Sugars and other sweet-tasting compounds are detected by the sweet taste receptor, a member of the class C GPCR family. The sweet receptor is a heterodimer composed of TAS1R2 and TAS1R3,3,4 two type 1 taste receptor family members that share the distinctive architecture of class C GPCRs: a large extracellular Venus flytrap (VFT) domain, responsible for ligand recognition; a cysteine-rich domain (CRD); and a seven-transmembrane (7TM) domain that mediates G protein coupling. To address this gap, here we present cryo-electron microscopy (cryo-EM) structures of the sweet receptor in the inactive, unliganded state, as well as in the activated, sucralose- and advantame-bound states. Unlike other class C GPCRs, such as mGluR, CaSR and GABAB receptors, where agonists stabilize inter-subunit VFT interactions to promote activation, the sweet receptor is activated by the rearrangement of a TAS1R2 VFT loop, which destabilizes interactions between the lower VFT lobes and the VFT–CRD interfaces.

We first determined the structure of the human/mouse sweet receptor in the absence of sweeteners. To improve the resolution, we combined all particles to generate a global reconstruction at 3.1 Å resolution, then performed local refinement focused on the VFT/CRD region or the 7TM domain, obtaining final resolutions of 2.9 Å and 3.6 Å, respectively. In the unliganded (apo) state, TAS1R2 and TAS1R3 show a highly asymmetric architecture, and their extracellular domains are markedly tilted relative to the membrane plane. In our apo sweet receptor structure, the two subunits pack closely against each other at both the upper and lower lobes of the VFT domains, as well as at the 7TM domains. This sharply contrasts with the apo states of mGluRs and the calcium-sensing receptor (CaSR), where the dimer interface is restricted to the VFT upper lobes (LB1s), while the lower lobes (LB2s) and 7TM domains remain largely disengaged. The tight packing of the sweet receptor is facilitated by interactions between VFT domains and CRDs, with the VFT LB2s held together by loops extending from the CRDs. Phe519 and His520 from TAS1R3 CRD are wedged deeply into the cleft between the two LB2s, effectively clasping them together, whereas equivalent residues Ile510 and His511 from TAS1R2 also extend into the VFT layer. This configuration reinforces the dimer interface and would enable the VFT domain of one subunit to directly communicate with the CRD of the other subunit, potentially allowing efficient cross-subunit allosteric coupling. Notably, such an arrangement differs from other class C GPCRs, where the VFT layer and the CRD remain structurally separated.

> SDFYLPGDYLLGGLFSLHANMKGIVHLNFLQVPMCKEYEVKVIGYNLMQAMRFAVEEINNDSSLLPGVLLGYEIVDVCYISNNVQPVLYFLAHEDNLLPIQEDYSNYSSRVVAVIGPDNSESVMTVANFLSLFLLPQITYSAISDELRDKVRFPALLRTTPSADHHIEAMVQLMLHFRWNWIIVLVSNDTYGRDNGQLLGERVARRGICIAFQETLPTLQPNQNMTSEERQRLVTIVDKLQQSTARVVVVFSPDLTLYHFFNEVLRQNFTGAVWIASESWAIDPVLHNLTELRHLGTFLGITIQSVPIPGFSEFREWGPQAGPPPLSRTSQSYTCNQECDNCLNATLSFNTILRLSGERVVYSVYSAVYAVAHALHSLLGCDKSTCTKRVVYPWQLLEEIWKVNFTLLDHQIFFDPQGDVALHLEIVQWQWDRSQNPFQSVASYYPLQRQLKNIQDISWHTINNTIPMSMCSKRCQSGQKKKPVGIHVCCFECIDCLPGTFLNHTEDEYECQACPNNEWSYQSETSCFKRQ;> LCLSQQFKAQGDYILGGLFPLGSTEEATLNQRTQPNSIPCNRFSPLGLFLAMAMKMAVEEINNGSALLPGLRLGYDLFDTCSEPVVTMKSSLMFLAKVGSQSIAAYCNYTQYQPRVLAVIGPHSSELALITGKFFSFFLMPQVSYSASMDRLSDRETFPSFFRTVPSDRVQLQAVVTLLQNFSWNWVAALGSDDDYGREGLSIFSSLANARGICIAHEGLVPQHDTSGQQLGKVLDVLRQVNQSKVQVVVLFASARAVYSLFSYSIHHGLSPKVWVASESWLTSDLVMTLPNIARVGTVLGFLQRGALLPEFSHYVETHLALAADPAFCASLNAELDLEEHVMGQRCPRCDDIMLQNLSSGLLQNLSAGQLHHQIFATYAAVYSVAQALHNTLQCNVSHCHVSEHVLPWQLLENMYNMSFHARDLTLQFDAEGNVDMEYDLKMWVWQSPTPVLHTVGTFNGTLQLQQSKMYWPGNQVPVSQCSRQCKDGQVRRVKGFHSCCYDCVDCKAGSYRKHPDDFTCTPCNQDQWSPEKSTACLPRR> GDVEEAIERAVVHVADTMRSGPSNSASVPALTAVETGHTSQVTPSDTMQTRHVKNYHSRSESTVENFLGRSACVYMEEYKTTDNDVNKKFVAWPINTKQMVQMRRKLEMFTYLRFDMEVTFVITSRQDPGTTLAQDMPVLTHQIMYVPPGGPIPAKVDDYAWQTSTNPSIFWTEGNAPARMSIPFISIGNAYSNFYDGWSNFDQRGSYGYNTLNNLGHIYVRHVSGSSPHPITSTIRVYFKPKHTRAWVPRPPRLCQYKKAFSVDFTPTPITDTRKDINTVTTVAQSRRRGDMSTLNTH;> SPTVEECGYSDRVRSITLGNSTITTQECANVVVGYGRWPTYLRDDEATAEDQPTQPDVATCRFYTLDSIKWEKGSVGWWWKFPEALSDMGLFGQNMQYHYLGRAGYTIHV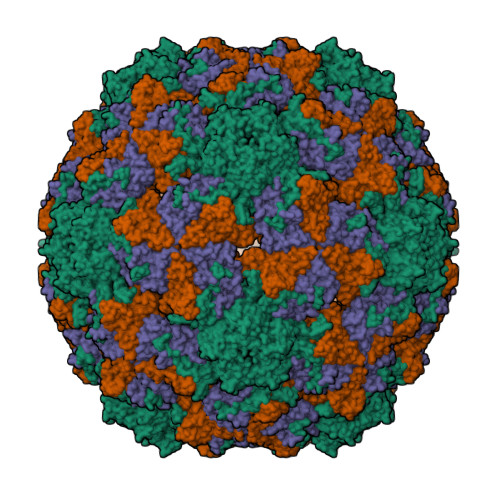QCNASKFHQGCLLVVCVPEAEMGGAVVGQAFSATAMANGDKAYEFTSATQSDQTKVQTAIHNAGMGVGVGNLTIYPHQWINLRTNNSATIVMPYINSVPMDNMFRHYNFTLMVIPFVKLDYADTASTYVPITVTVAPMCAEYNGLRLAQAQ;> GLPTMNTPGSTQFLTSDDFQSPCALPQFDVTPSMNIPGEVKNLMEIAEVDSVVPVNNVQDTTDQMEMFRIPVTINAPLQQQVFGLRLQPGLDSVFKHTLLGEILNYYAHWSGSMKLTFVFCGSAMATGKFLIAYSPPGANPPKTRKDAMLGTHIIWDIGLQSSCVLCVPWISQTHYRLVQQDEYTSAGYVTCWYQTGMIVPPGTPNSSSIMCFASACNDFSVRMLRDTPFISQDNKLQ> MGSDRSCVLSVF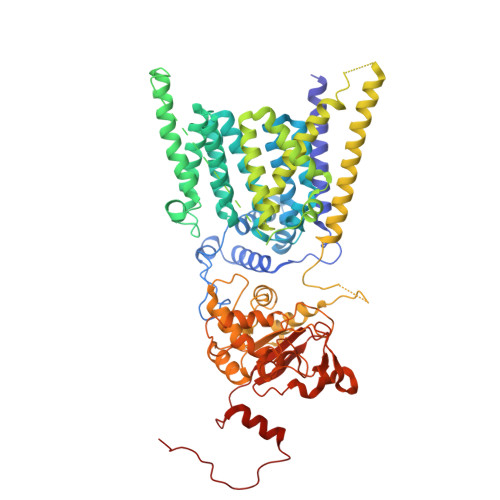QTILKLVIFVAIFGAAISSRLFAVIKFESIIHEFDPWFNYRATKYLVNNSFYKFLNWFDDRTWYPLGRVTGGTLYPGLMTTSAFIWHALRNWLGLPIDIRNVCVLFAPLFSGVTAWATYEFTKEIKDASAGLLAAGFIAIVPGYISRSVAGSYDNEAIAITLLMVTFMFWIKAQKTGSIMHATCAALFYFYMVSAWGGYVFITNLIPLHVFLLILMGRYSSKLYSAYTTWYAIGTVASMQIPFVGFLPIRSNDHMAALGVFGLIQIVAFGDFVKGQISTAKFKVIMMVSLFLILVLGVVGLSALTYMGLIAPWTGRFYSLWDTNYAKIHIPIIASVSEHQPVSWPAFFFDTHFLIWLFPAGVFLLFLDLKDEHVFVIAYSVLCSYFAGVMVRLMLTLTPVICVSAAVALSKIFDIYLDFKTSDRKYAIKPAALLAKLIVSGSFIFYLYLFVFHSTWVTRTAYSSPSVVLPSQTPDGKLALIDDFREAYYWLRMNSDEDSKVAAWWDYGYQIGGMADRTTLVDNNTWNNTHIAIVGKAMASPEEKSYEILKEHDVDYVLVIFGGLIGFGGDDINKFLWMIRISEGIWPEEIKERDFYTAEGEYRVDARASETMRNSLLYKMSYKDFPQLFNGGQATDRVRQQMITPLDVPPLDYFDEVFTSENWMVRIYQLKKDDAQGRTLRDVGELTRSSTKTRRSIKRPELGLRV> GDPVEDIIHDALGNTARRAISSATNVESAANTTPSSHRLETGRVPALQAAETGATSNATDENMIETRCVVNRNGVLETTINHFFSRSGLVGVVNLTDGGTDTTGYATWDIDIMGFVQLRRKCEMFTYMRFNAEFTFVTTTENGGARPYMLQYMYVPPGAPKPTGRDAFQWQTATNPSVFVKLTDPPAQVSVPFMSPASAYQWFYDGYPTFGQHPETSN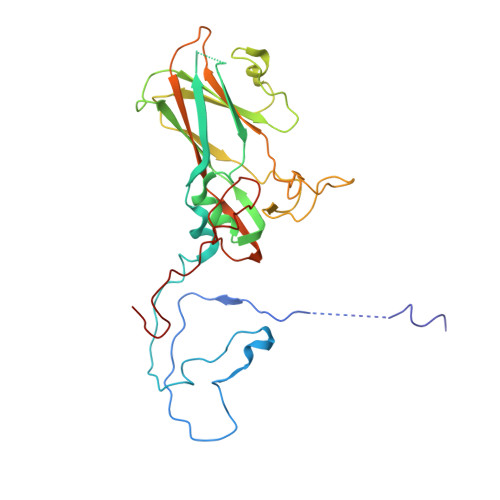TTYGLCPNNMMGTFAVRVVSREASQLKLQTRVYMKLKHVRAWVPRPIRSQPYLLKNFPNYDSSKITNSARDRSSIKQANM cyclobutyl[(3aS,4R,5R,7S,8aS)-4,5-dihydroxyhexahydro-1H-3a,7-epoxycyclohepta[c]pyrrol-2(3H)-yl]methanone | C14 H21 N O4 | 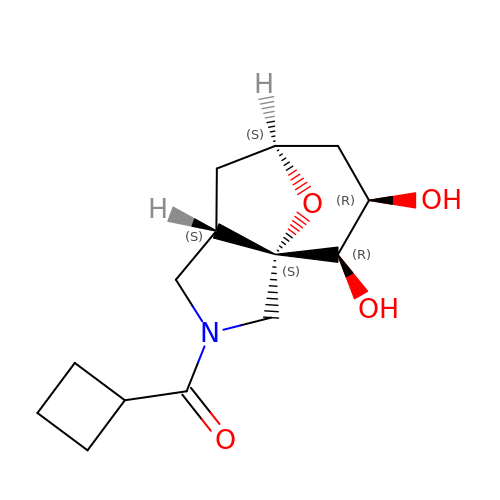BYVLFJJVWOHEND-JCCXBDGPSA-N> MTNLQDQTQQIVPFIRSLLMPTTGPASIPDDTLEKHTLRSETSTYNLTVGDTGSGLIVFFPGFPGSIVGAHYTLQGNGNYKFDQMLLTAQNLPASYNYCRLVSRSLTVRSSTLPGGVYALNGTINAVTFQGSLSELTDVSYNGLMSATANINDKIGNVLVGEGVTVLSLPTSYDLGYVRLGDPIPAIGLDPKMVATCDSSDRPRVYTITAADDYQFSSQYQPGGVTITLFSANIDAITSLSVGGELVFRTSVHGLVLGATIYLIGFDGTTVITRAVAANNGLTTGTDNLMPFNLVIPTNEITQPITSIKLEIVTSKSGGQAGDQMSWSARGSLAVTIHGGNYPGALRPVTLVAYERVATGSVVTVAGVSNFELIPNPELAKNLVTEYGRFDPGAMNYTKLILSERDRLGIKTV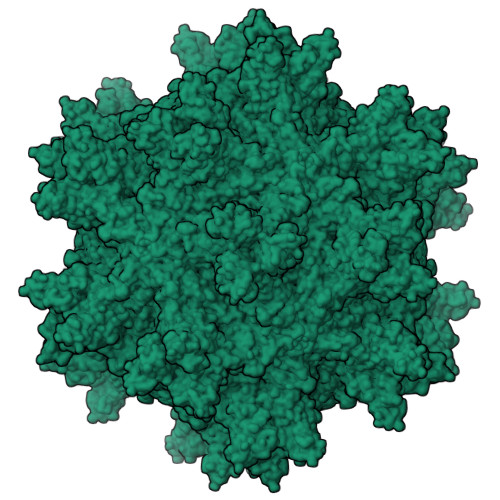WPTREYTDFREYFMEVADLNSPLKIAGA In bacteria, however, a different strategy employing a class of enzyme known as polysaccharide lyases (PL) is deployed. PLs selectively target glycans composed of uronic acids with a C4 hydroxyl group linked to the preceding sugar in the glycan chain. This enables PLs to operate through a β-elimination mechanism that relies on proton abstraction from the C5 carbon of the uronic acid sugar ring, resulting in double bond formation between C4 and C5 and elimination of the preceding sugar. The three characterized PL33_1 enzymes were all from Bacteroides species inhabiting the human colon: BT4410 (BtPL33HA) and BcellWH2_04512 (BcPL33HA) are hyaluronidases from Bacteroides thetaiotaomicron VPI-5482 (B. theta) and Bacteroides cellulosilyticus WH2 (B. cell), respectively, while HMPREF1181_01744 (BsPL33Heparosan) is a heparosanase from Bacteroides stercoris CC31F (B. stercoris). The enzymes are 68% identical and contain a larger N-terminal α-helical (α/α)6 toroid domain (residues 21 to 401; BtPL33HA numbering used throughout this section unless specified) and a smaller β-sheet C-terminal domain (residues 402 to 635).

Based on the Apo structures of BtPL33HA and BcPL33HA, combined with Consurf analysis, a total of 20 BtPL33HA mutants were made in order to understand the roles of individual amino acids in substrate binding and catalysis. This enabled the structural characterization of a catalytically compromised variant (Y291A) of BtPL33HA in complex with a HA tetrasaccharide. The complex contained two molecules of BtPL33HA in the asymmetric unit, with one molecule containing electron density for which a trisaccharide could be modeled, and the other for which a less well-ordered tetrasaccharide could be modeled. A hydrophobic platform composed of W224, W239, L174, and W242 underpins binding at the +2, +1, and −1 subsites, while no obvious interactions occur with the −2 sugar. The +1 subsite, the site of catalysis, is where the majority of interactions occur. The side chain of R103 interacts with the O2 and O3 of the +1 GlcA, while H154 only interacts with O2. N238 interacts with the carboxylate of the +1 GlcA through its amide group, while Y291 lies ~6 Å from C5. No activity could be quantified for the mutants N238A or Y291A. However, it should be noted that although both Y291 and H444 are positioned below the beta face of the +1 GlcA, they are too remote to directly abstract a proton from C5. Furthermore, N238 coordinates with the carboxyl group from above the alpha face, suggesting a role in charge stabilization rather than proton abstraction. This suggests significant conformational shifts are needed for Y291 and H444 to perform a direct role in catalysis.

>[2x]MGSSHHHHHHSSGLVPRGSHMASNAYTERDMLQKAADETTLKNVLVMKQAWVPYPAYTDRAAWDSLMGSNKQRLIAAGEKLLDYKWQLIPATAYLEYERTGNRKIMEVPYDANRQALNTLMLAELAEGKGRFIDQLLNGAYMSCEMNSWVLSAHLPRQSSKRSLPDFREQIIDLGSGGYGALMAWVHYFFRKPFDKINPVVSLQMRKAIKERILDPYMNDDDMWWMAFNWQPGEIINNWNPWCNSNALQCFLLMENNKDRLAKAVYRSMKSVDKFINFVKSDGACEEGTSAWGHAAGKLYDYLQILSDGTGGKISLLNEPMIRRMGEYMSRSYVGNGWVVNFADASAQGGGDPLLIYRFGKAVNSNEMMHFAAYLLNGRKPYATMGNDAFRSLQSLLCCNDLAKETPKHDMPDVTWYPETEFCYMKNKNGMFVAAKGGFNNESHNHNDVGTFSLYVNTIPVILDAGVGTYTKQTFGKDRYTIWTMQSNYHNLPMINGIPQKYGQEYKATNTTCNEKKRVFSTDIAAAYPSEAKVKNWIRSYTLDDRKLTITDSYTLEEAVAPNQVNFMTWGNVTFPSQGKIQIEVKGQKVELDYPTLFKAELETIQLDDPRLSNVWGKEIYRITLKTNEKKETGNYKFVIQQIK> GVGPVADNTITNAATSPDGFSRQAVVVNGVTPGPLVAGNIGDRFQLNVIDNLTNHTMLKTTSVHWHGFFQQGTNWADGPAFINQCPISPGHSFLYDFQVPNQAGTFWYHSHLSTQYCDGLRGPFVVYDP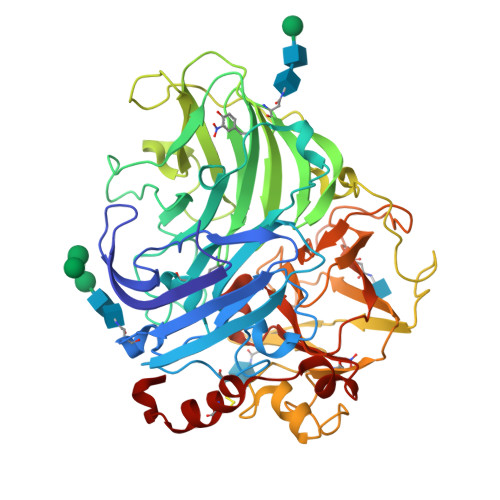NDPHASRYDVDNDDTTITLADWYHTAAKLGPAFPNGADSTLINGKGRAPSDSSAQLSVVSVTKGKRYRFRLVSLSCDPNFTFSIDGHNNTIIETDSVNSQPLNTDSIQIFAAQRYSFTLNANQAVDNYWIRANPNFGNVGFNGGINSAILRYDGAPAVEPTTNQSTSTQPLNETNLHPLVSTPVPGSPAAGGVDKAINMAFNFNGSNFFINGASFTPPSVPVLLQILSGAQTAQDLLPSGSVYTLPSNASIEISFPATAAAPGAPHPFHLHGHVFAVVRSAGSTVYNYSNPIFRDVVSTGTPAAGDNVTIRFLTNNPGPWFLHCHIDFHLEGGFAVVQAEDVPDVKATNPVPQAWSDLCPTYDANAPSDQ>MSMPRYYEYRHVVGFEETNLVGNVYYVNYLRWQGRCREMFLYEHAPEILDELRADLKLFTLKAECEFFAELAPFDRLAVRMRLVELTQTQMELGFDYLRLGGDDLLVARGRQRIACMRGPNGRTEPVRVPA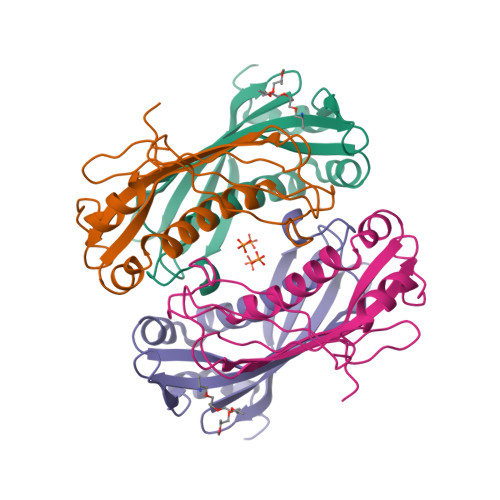GLVRAFAPFRSATVGQ[6x]>[2x]GPMSDQVSLGVVGIGKIARDQHLPAIDAEPGFKLTACASRHAEVTGVRNYRDLRALLAAERELDAVSLCAPPQVRYAQARAALEA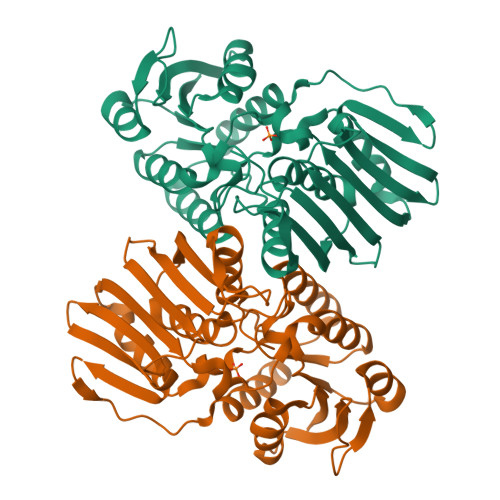GKHVMLEKPPGATLGEVAVLEALARERGLTLFATWHSRCASAVEPAREWLATRAIRAVQVRWKEDVRRWHPGQQWIWEPGGLGVFDPGINALSIVTRILPRELVLREATLIVPSDVQTPIAAELDCADTDGVPVRAEFDWRHGPVEQWEIAVDTADGVLAISRGGAQLSIAGEPVELGPEREYPALYAHFHALIARGESDVDVRPLRLVADAFLFGRRVQTDAFGR> GPL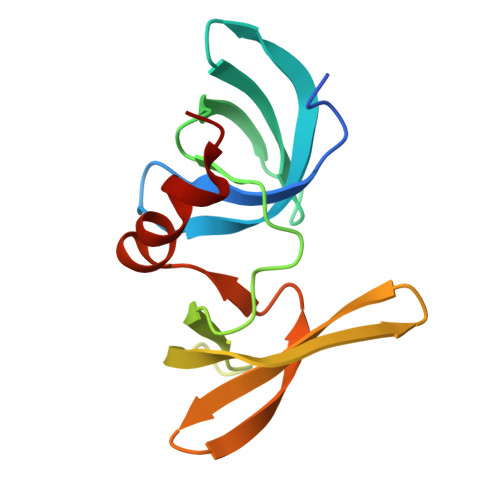GSNSFVGLRVVAKWSSNGYFYSGKITRDVGAGKYKLLFDDGYECDVLGKDILLCDPIPLDTEVTALSEDEYFSAGVVKGHRKESGELYYSIEKEGQRKWYKRMAVILSLEQGNRLREQYGLG>MGSDKIHHHHHHMKNLVVVDHPLIKHKLTIMRDKNTGPKEFRELLREITLLLAYEATRHLKCEEVEVETPITKTIGYRINDKDIVVVPILRAGLVMADGILELLPNASVGHIGIYRDPETLQAVEYYAKLPPLNDDKEVFLLDP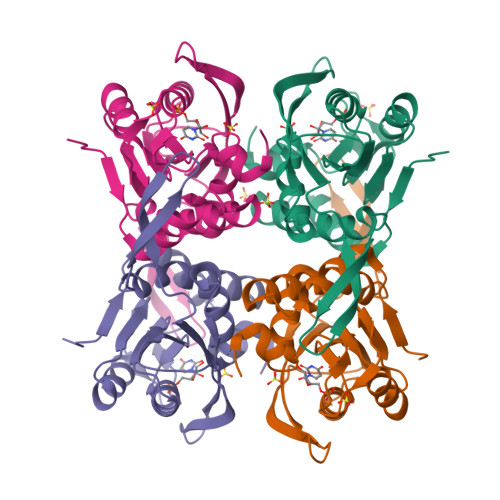MLATGVSSIKAIEILKENGAKKITLVALIAAPEGVEAVEKKYEDVKIYVAALDERLNDHGYIIPGLGDAGDRLFRTK[4x]>TPEGLSSEQQRAFLAVTQTPHPAHLITGPAGTGKTTLLYALQKFYKCRAVTLAPTGTAALQARGQTVHSFFRFPARLLRYRHPEDIRPPGPHSPLRKAIEQMEVLILDEVGMVRVDLLEAMDWALRKTRKRLEEPFGGVKVLLLGDTRQLEPVVPGGEEALYIARTWGGPFFFQAHVWEEVALRVHRLWESQRQREDPLFAELLKRLRQGDPQALETLNRAAVRPDGGEEPGTLILTPRRKEADALNLKRLEALPGKPLEYQAQVKGEFAETDFPTEAALTLKKGAQVILLRNDPLGEYFNGDLGWVEDLEAEALAVRLKRNGRRVVIRPFVWEKIVYTYDSEREECKPQVVGTFRQVPVRLAWALTVH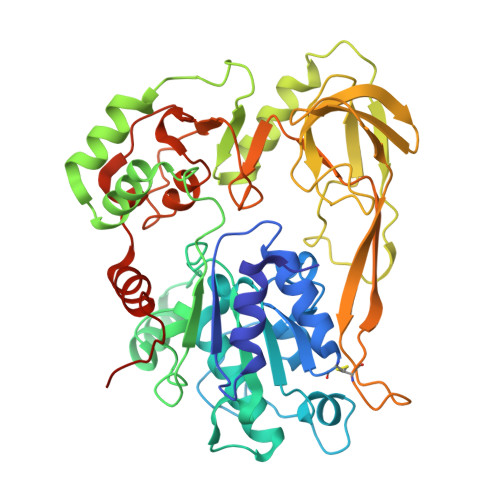KAQGLTLDKVHLELGRGLFAHGQLYVALTRVRRLQDLSLSRPIAPTELLWRPEVEVFETRIQEGIWQKSHGWPSLVD[2x]>[10x]MSVLDELYREILLDHYQSPRNFGVLPQATKQAGGMNPSCGDQVEVMVLLEG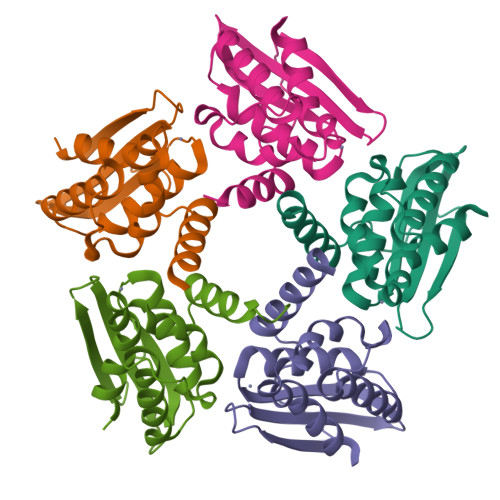DTIADIRFQGQGCAISTASASLMTEAVKGKKVAEALELSRKFQAMVVEGAPPDPTLGDLLALQGVAKLPARVKCATLAWHALEEALR>GPHMMSGEKRVLSGRVAVVTGSTSGIGLGIAMRLAMAGADVVLNGRRQSPEDSAIVEKVAAYGTRVRYFAANMKDRAQVEALIKFTEKELGAVEILVNNAGIQHVSPVETFPSDKWDEIIALNLTSAFHATQLCLPSMRQRGWGRIINIASVQGLVGSMNKSAYCAAKHGLIGFTKVVALETATTGI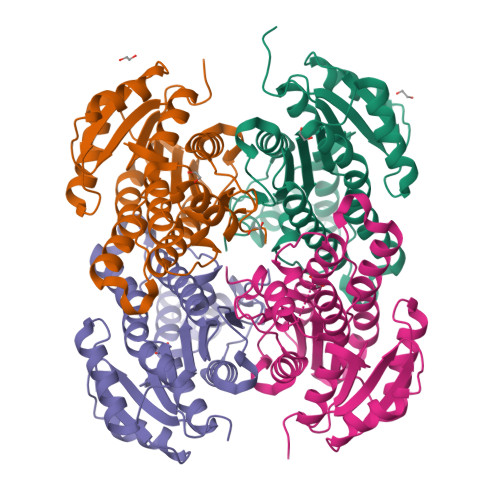TCNAICPGYVYTPLVEEQIKAVAEAKYGGDMEAATQAFLCEKQPAKAFVTVEQVGDAAVFLASPGADMIRGTTITVDGGWVAQ[4x]> MHHHHHHGSMSDM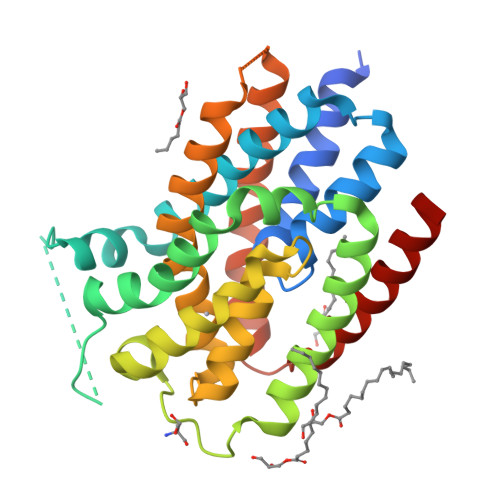HSLLIAAILGVVEGLTEFLPVSSTGHMIIVGHLLGFEGDTAKTFEVVIQLGSILAVVVMFWRRLFGLIGIHFGRPLQHEGESKGRLTLIHILLGMIPAVVLGLLFHDTIKSLFNPINVMYALVVGGLLLIAAECLKPKEPRAPGLDDMTYRQAFMIGCFQCLALWPGFSRSGATISGGMLMGVSRYAASEFSFLLAVPMMMGATALDLYKSWGFLTSGDIPMFAVGFITAFVVALIAIKTFLQLIKRISFIPFAIYRFIVAAAVYVVFF> AHIEGRHMKRMLINATQQEELRVALVDGQRLYDLDIESPGHEQKKANIYKGKITRIEPSLEAAFVDYGAERHGFLPLKEIAREYFPANYSAHGRPNIKDVLREGQEVIVQIDKEERGNKGAALTTFISLAGSYLVLMPNNPRAGGISRRIEGDDRTELKEALASLELPEGMGLIVRTAGVGKSAEALQWDLSFRLKHWEAIKKAAESRPA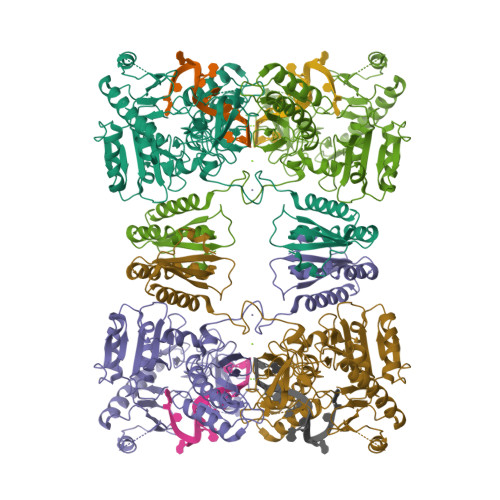PFLIHQESNVIVRAFRDYLRQDIGEILIDNPKVLELARQHIAALGRPDFSSKIKLYTGEIPLFSHYQIESQIESAFQREVRLPSGGSIVIDSTEALTAIDINSARATRGGDIEETAFNTNLEAADEIARQLRLRDLGGLIVIDFIDMTPVRHQRAVENRLREAVRQDRARIQISHISRFGLLEMSRQRLSPSLGESSHHVCPRCSGTGTVRDNESLSLSILRLIEEEALKENTQEVHAIVPVPIASYLLNEKRSAVNAIETRQDGVRCVIVPNDQMETPHYHVLRVRKGEETPTLSYMLPKLHEEAM>MAHHHHHHDMAGVKALVTAGGTREPLDPVRFIGNRSSGKQGYAVARVLAQRGADVTLIAGNTAGLIDPAGVEMVHIGSATQLRDAVSKHAPDANVLVMAAAVADFRPAHVAAAKIKKGASEPSSIDLVRNDDVLAGAVRARADGQLPNMRAIVGFAAETGDANGDVLFHARAKLERKGCDLLVVNAVGENRAFEVDHNDGW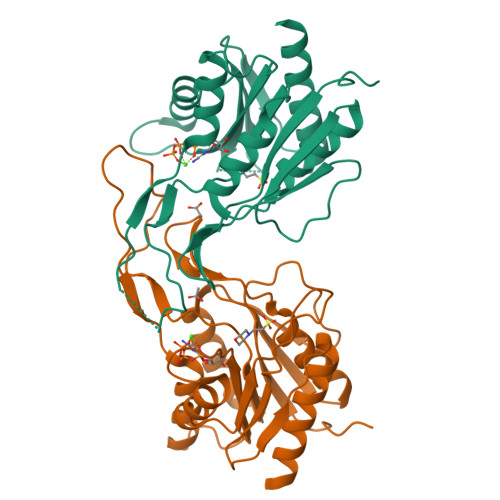LLSADGTESALEHGSKTLMATRIVDSIAAFLKSQDG[4x]>[4x]SMSSSDRAMMNAFKEITTMADRINLPRNIVDRTNNLFKQ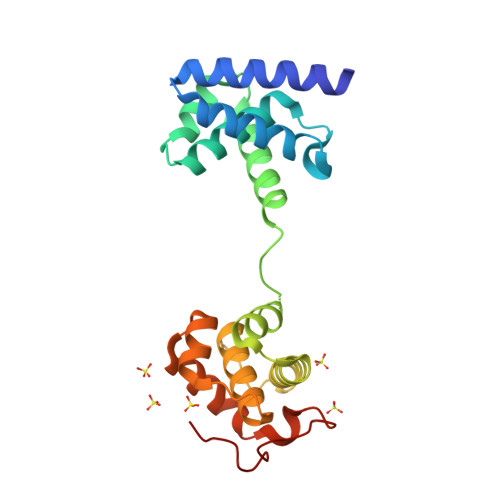VYEQKSLKGRANDAIASACLYIACRQEGVPRTFKEICAVSRISKKEIGRCFKLILKALETSVDLITTGDFMSRFCSNLCLPKQVQMAATHIARKAVELDLVPGRSPISVAAAAIYMASQASAEKRTQKEIGDIAGVADVTIRQSYRLIYPRAPDLFPTDFKFDTPVDKLPQL>MGSSHHHHHHSSGLVPRGSHQHSSVLVKSASTQMLDESARLRLEARGELQALRIQRYFMDAFQYGKGFSRQILFLRDQAQKRFLDAYDLREDLTRQVRTALAANPEVLGLYVVFEPNALDGKDELFVDQPALGSNDKGRFSLYWAQATPGQLESESMIESELADTSSGPSGAAYNAWYTCPKESGQPCVLDPYFDKVGERQLLMTSIAFPLELDGKVIGVMGLDINLSNLQALSEQGNRELYDGVGQVGILSPAGLFAGNSRDAGLLGKNLAKADPQHAGELLQLLAAGKSRLFNENDDLKVLQPLQPIPGAKPWGVLLEVPKSALLGPALALERQLDDMRREGT[4x]

Here, we report that the opportunistic human pathogen Pseudomonas aeruginosa exhibits chemotaxis toward histamine. This chemotactic response is mediated by the concerted action of the TlpQ, PctA, and PctC chemoreceptors, which display differing sensitivities to histamine. TlpQ is the first bacterial histamine receptor to be described and greatly differs from human histamine receptors, indicating that eukaryotes and bacteria have pursued different strategies for histamine recognition. High sensitivity histamine responses are mediated by the TlpQ chemoreceptor, which binds histamine directly.

To determine the molecular determinants for histamine recognition by TlpQ, we solved the high-resolution structure of TlpQ-LBD in complex with histamine. There are four monomers in the asymmetric unit,and the superimposition of their Cα atoms resulted in root mean square deviation (RMSD) values of 0.4 to 0.8 Å, indicative of high similarity. An inspection of the structure revealed that it is a dCACHE domain. A long N-terminal helix is followed by two globular α/β modules, termed membrane-proximal and membrane-distal modules. The membrane-distal module contained bound histamine in all four monomers of the asymmetric unit. Of all the homologous domains that we identified, TlpQ-LBD was the largest, at 334 amino acids, namely due to particularly long inserts between β-strands 1 and 2, extended helices α1 and α2, and an extended loop between helices η3 and α3. TlpQ ligands are present as protonated polycations at neutral pH, which explains why the ligand binding pocket is highly negatively charged. TlpQ ligands contain at least one primary amino group, and the primary amino group of histamine plays a central role in binding because it forms hydrogen bonds with the side chains of Tyr208, Asp210, and Asp239. In addition, this histamine amino group interacts with a water molecule coordinated by the main chain oxygen of Lys211 and the hydroxyl group of Tyr158. Each of the histamine imidazole nitrogen atoms forms hydrogen bonds with Asp210 and Glu170.> MSKILVIAEHRR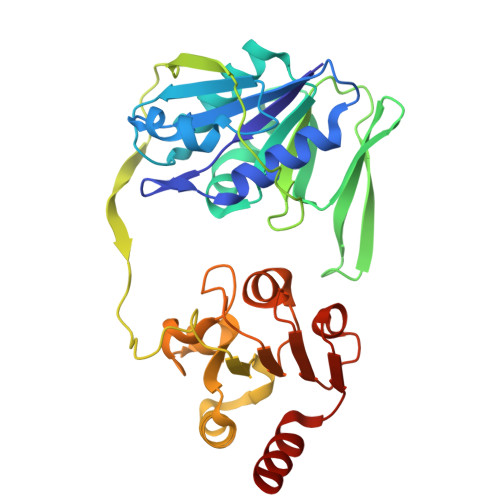NDLRPVSLELIGAANGLKKSGEDKVVVAVIGSQADAFVPALSVNGVDELVVVKGSSIDFDPDVFEASVSALIAAHNPSVVLLPHSVDSLGYASSLASKTGYGFATDVYIVEYQGDELVATRGGYNQKVNVEVDFPGKSTVVLTIRPSVFKPLEGAGSPVVSNVDAPSVQSRSQNKDYVEVGGGNDIDITTVDFIMSIGRGIGEETNVEQFRELADEAGATLCCSCPIADAGWLPKSRQVGQSGKVVGSCKLYVAMGISGSIQHMAGMKHVPTIIAVNTDPGASIFTIAKYGIVADIFDIEEELKAQLAA> MLQKKPYNGLHEKELNQINQQDGSPCVAISAPGCFIKGSNLFSEKRAGNRVRFFTTGRDYFSDLASALDSASSSIFITGWQVNYDVLLDGRRSLWQCLRQALERSPALKVYVMPWLSPSGSLGTYDFETMLAVFQLNAGLEGGARAFCTPAIQQSDMQGLGVAFSHHQKSVVIDNRIGYVGGIDLAYGRRDDNDFSLDASGRRGNDAYNPGLPHLGWMAEDEHVSSMGLMMATLFDLSRPLASLTLHAPTLRLSPFPHIAASDEPLLSIPLAPSRARALNGAAYLSDLFRSPMLPSLQWLGRAYNSSKEGLDEGFERLDALRRQMVASSIRAIANLIADNLDALPIEPELERRLRAWLEELRTAALNLPEALRIKSLLLINQWMSETELGQVLTLISGKGFEDIPQNLSGKAGELAGSLFWTLHRLMQARAGGHQQPYRYLDEAPQPLASPDNARLAADQPRMPWQDVHCRIEGPSVYDLARNFIDRWNGQQAYLAKTPALQDTALVRSALEAVMKWLNSLAAAAGLENYLDEKRNLRLELDPPTPCWINAPEQLPQEPEVRRGGMTVQVLRSAAARMLEQEQAGRLGAGVNLPLQVGVSTEGVQSNCKDAMLLAISGAQQFIYIENQFFQSEFGKEGEVFKDLPLSGPMASLRDVGSLRRDFVVRIRLEEALEQRDLWLLDWAEVEKIAQEPGTEARQFLKSMLAMWGVNAQGWLTHKLGEAQHGLLNEIGEALARRIERAIQREHPFHVYLVLPVHPEGALNVPNIMHQVHLTQQSLVFGEQSLVKRIQRQMALKALEGKSDPAQAREIIERKDARGRPVYEQQDWSRYLTLLNLRTWAVLGGRVVTEQIYVHSKLLIADDRVAILGSANINDRSLQGERDSELAVMVRDSEPLTVRLDGKNDAIVGKAIHQLRVNLWKKHFGLSQGPGGFVKPASELSAYLSIPAAQEAWEAIQTLAKENTRAYERTFNFIPQNISQTQLQLTPEPPKGFEDGFPASIWPTWAYRKPGELRAGGQLMEPMPYQEIFWRSSNLTSVKTFPPPNGVSGFITALPTSWTRGERNDSGLNLSILAHQDSRSLPTQVAMNGDSSAQGKHRT;> MKRVLMGLILLSSSNITWAEAPSSKYQECLGRMTFEIPEEMEWATYDASRVWQISKGGGHNFTAEVTAVGDNGSYDYDSMIFYVSEKVDKNEFHNASNYIKGTAEIYQDHLRENIKLDKKAISTLQKNKSEEKSIERIKKGIAEMEAKIPLAKIYEHDLGIPDSHILGSKNIPFHVLLWRNQRVYYFTFSKPTENSAQRIKDLIARFRTRELYEVPNEPGICFPYGFIADDGKTAYELKNSLRFTRTPNVIFSLLTASANDPWQTRPTSGLYDSDFRPGYDRQKWKKSALLDSLHIGKRLAAFEGWRLDPRPDSGERERAWFGLAHTGGTLDPLVAIQVQTFQKGTDDLTDYTPPPEEVLPRLKALSQSIEQRLAR

PldA, a phospholipase D (PLD) effector, catalyzes hydrolysis of the phosphodiester bonds of glycerophospholipids—the main component of cell membranes—and assists the invasion of the opportunistic pathogen Pseudomonas aeruginosa. As a cognate immunity protein, PA3488 can inhibit the activity of PldA to avoid self-toxicity. PldA is mainly composed of 27 α-helices, 25 β-strands, twelve 310 helices, and many loops, folding into three regions: the core catalytic domain (CCD, aa 24–935), the peripheral helical domain (PD, aa 215–441 + aa 647–721), and a small C-terminal domain (CTD, aa 936–1094). Compared to the open conformation exhibited by PldAFL (pre-open state), PldAtruncate presents a highly open conformation (open state) and the PA3488-inhibited PldA reveals an almost closed conformation (pre-closed state).

To understand the structural basis of the intrinsic activity of PldA and the way in which PA3488 inactivates PldA, we next determined the cryo-EM structure of the PldA–PA3488 complex by single-particle analysis with a resolution of 3.05 Å. The structure of the PldA–PA3488 complex indicates that both proteins tightly interact with each other, burying a ~2020 Å2 solvent-accessible surface area, and PA3488 acts like a crab claw to clamp the HKD2 and CTD domains of PldA. Four interfaces participate in the formation of the PldA–PA3488 complex. The specificity of binding is due primarily to a salt bridge between the Asp643 of PldA and Arg50 of PA3488, combined with complementary van der Waals interactions between the Asp643 of PldA and the Gly70 of PA3488. The results suggested that PldAD643A and PA3488R50A dramatically decrease the PldA–PA3488 interaction, which is consistent with their functions in stabilizing the PldA–PA3488 complex through forming a tight salt bridge. In contrast, in the inhibited PldA, on account of the binding of PA3488, the 310 helix melts, allowing the region to instead form an extended loop, stretching out and following the α3 helix direction and resulting in the formation of a shorter α3 helix than that of apo-PldA. This is associated with a translation of the lid toward the active site and a rotation of roughly 140° (based on Cα of Ser121), so that the backbone atoms in the lid region are as much as 4.8 Å away from their counterparts in PldAFL. On binding PA3488, the whole lid region slightly changes its position and orientation with respect to the active site, sitting on the top of it and almost entirely occluding the entrance of the solvent and substrate. Coincidently, activity assays showed that the PldA almost but not completely lost its enzyme activity upon PA3488 binding; hereafter, we refer to PA3488-inhibited PldA as “pre-closed” PldA. Of note, the α5-α8 loop of the PD1 domain in the inhibited PldA is structurally invisible in the electron microscopy map, implying that these helices are highly dynamic after PA3488 binding, and this accordingly imparts flexibility to the lid region.>[2x]SNAMTLLDGKALSAKIKEELKEKNQFLKSKGIESCLAVILVGDNPASQTYVKSKAKACEECGIKSLVYHLNENITQNELLALINTLNHDDSVHGILVQLPLPDHICKDLI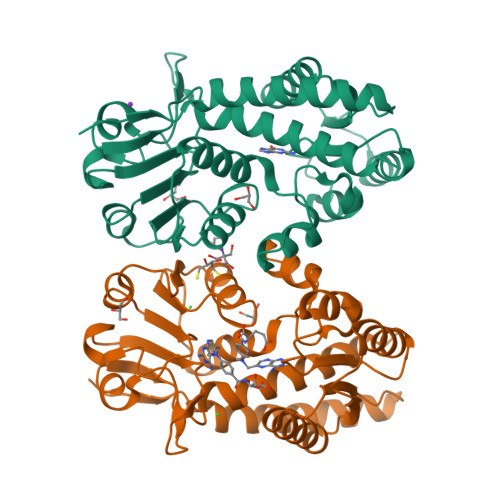LESIISSKDVDGFHPINVGYLNLGLESGFLPCTPLGVMKLLKAYEIDLEGKDAVIIGASNIVGRPMATMLLNAGATVSVCHIKTKDLSLYTRQADLIIVAAGCVNLLRSDMVKEGVIVVDVGINRLESGKIVGDVDFEEVSKKSSYITPVPGGVGPMTIAMLLENTVKSAKNRLN Here we report the discovery of a natural protein, citrate synthase from the cyanobacterium Synechococcus elongatus, which self-assembles into Sierpiński triangles. Bacterial citrate synthase (CS) proteins are homo-oligomeric enzymes that can assemble into dimers and hexamers. CS catalyses the condensation of acetyl-CoA and oxaloacetate to citrate as the first step in the tricarboxylic acid cycle. Using cryo-electron microscopy, we reveal how the fractal assembles from a hexameric building block.

We were led in this direction because fractal complexes are pH sensitive. Indeed, an increase in the pH from 7.5 to 9 led to complete disassembly of the structure into hexamers. This behaviour is driven by the residue H369 in the fractal interface, and changing it to arginine abolished the pH sensitivity without compromising its assembly into fractals. Instead, we solved this structure for a point mutant (H369R), which we generated in the course of a structure–function analysis (described further below). This protein also forms 18mers at levels that are indistinguishable from wild-type SeCS at 50 nM. Moreover, it is capable of forming the larger assemblies.

>MTAVSEFRPGLEGVPATLSSISFVDGQRGVLEYRGISIEQLAQQSSFLETAYLLIWGHLPTQQELTEFEHEIRYHRRIKFRIRDMMKCFPDSGHPMDALQASAAALGLFYSRRALDDPEYIRAAVVRLLAKIPTMVAAFQLIRKGNDPIQPRDELDYAANFLYMLTEREPDPVAARIFDICLTLHAEHTINASTFSAMVTASTLTDPYAVVASAVGTLAGPLHGGANEEVLDMLEAIGSVENVEPYLDHCIATKTRIMGFGHRVYKVKDPRAVILQNLAEQLFDIFGHDPYYEIAVAVEKAAAERLSHKGIYPNVDFYSGLVYRKLGIPSDLFTPVFAIARVAGWLAHWKEQLNENRIFRPTQIYTGSRNLDYTPIADRDLAIESDLEHHHHHH[18x]> MGVEKVPKYDIPTKKVDYVFIELDKMKPHEQLVQKELEAFIESVTGSGIFWKPMLLAKVPGEDMYLIVDGHHRWAGLQKLGAKRAPSVILDYFSDDVKVYTWYPAFKGDLNEVVERLKKEGLEVIEDPEAEEKAERGEIAFALVGEKSFAIPGG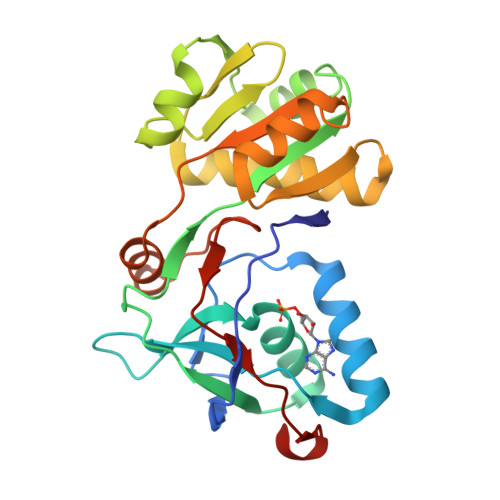LEEQKKVSKVLDEMSVEGKIELIYYGLKEDAREDMAKGEIDYVFIRKAPTKEEVMELVKRGEVYSPKTTRHVLPFNPDKIDVKLEELF but-3-yn-1-yl trihydrogen diphosphate | C4 H8 O7 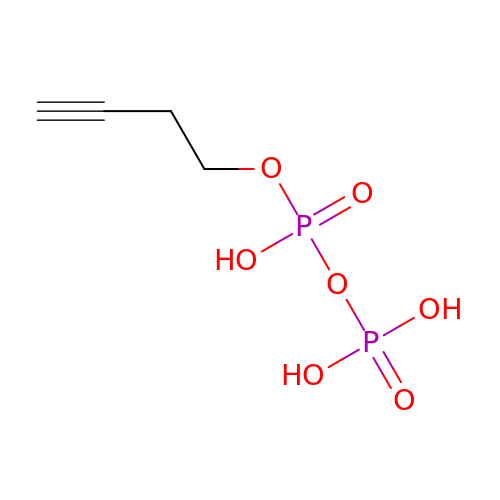P2 | GYFWQGOZWDTPGX-UHFFFAOYSA-N> ANDPFTIVHGNTGKCIKPVYGWIVADDCDETEDKLWKWVSQHRLFHLHSQKCLGLDITKSVNELRMFSCDSSAMLWWKCEHHSLYGAARYRLALKDGHGTAISNASDVWKKGGSEESLCDQPYHEIYTRDGNSYGRPCEFPFLIDGTWHHDCILDEDHSGPWCATTLNYEYDRKWGICLKPENGCEDNWEKNEQFGSCYQFNTQTALSWKEAYVSCQNQGADLLSINSAAELTYLKEKEGIAKIFWIGLNQLYSARGWEWSDHKPLNFLNWDPDRPSAPTIGGSSCARMDAESG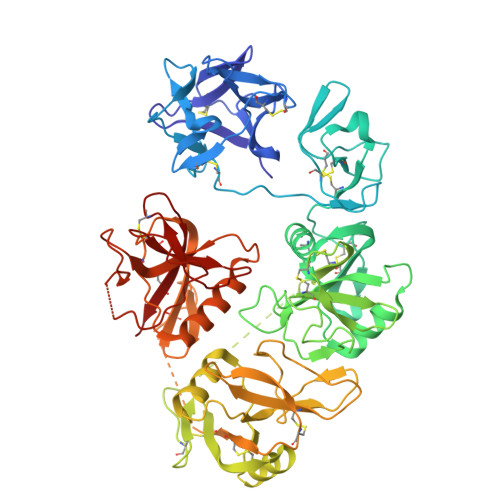LWQSFSCEAQLPYVCRKPLNNTVELTDVWTYSDTRCDAGWLPNNGFCYLLVNESNSWDKAHAKCKAFSSDLISIHSLADVEVVVTKLHNEDIKEEVWIGLKNINIPTLFQWSDGTEVTLTYWDENEPNVPYNKTPNCVSYLGELGQWKVQSCEEKLKYVCKRKGEKLNDASSDKMCPPDEGWKRHGETCYKIYEDEVPFGTNCNLTITSRFEQEYLNDLMKKYDKSLRKYFWTGLRDVDSCGEYNWATVGGRRRAVTFSNWNFLEPASPGGCVAMSTGKSVGKWEVKDCRSFKALSICKKMS>[2x]G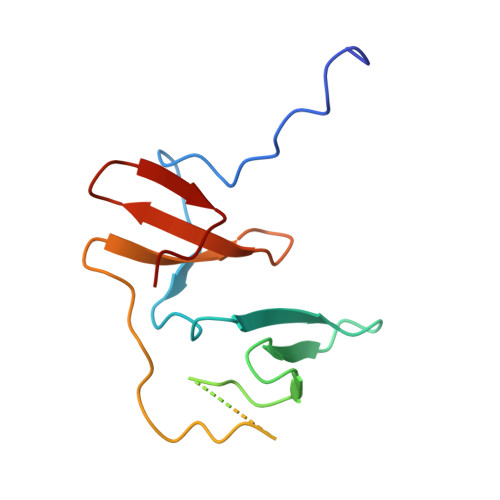PGSDRPPPYVAPPSYEGPHRTLGVPLPAGWEMAKTSSGQRYFLNHNDQTTTWQDPRKAMLSQLNVPAPASPAVPQTLMNSASGPLPDGWEQAMTQDGEVYYINHKNKTTSWLDPR> GAMSRQANRGTESKKMSSELFTLTYGALVTQLCKDYENDEDVNKQLDRMGYNIGVRLIEDFLARSNVGRCHDFRETADVIAKVAFKMYLGITPSITNWSPAGDEFSLILENNPLV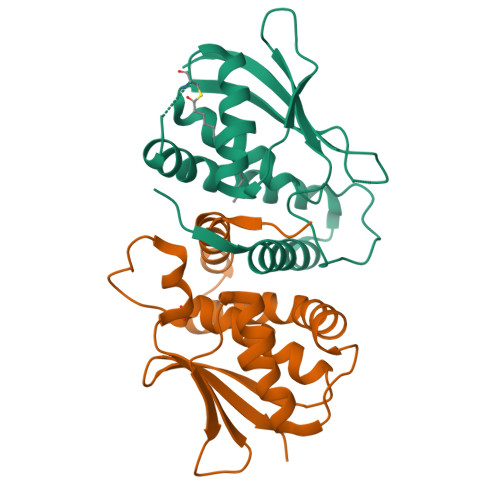DFVELPDNHSALIYSNLLCGVLRGALEMVQMAVEAKFVQDTLKGDGVTEIRMRFIRRIEDNLPAGEE;> PKTEVSVSAFALLFSEMVQYCQSRVYSVSELQARLADMGQGVGASLLDVLVMREKNGKRETKVLNILLFIKVNVWKALFGKEADKLEQANDDDKTYYIIEKEPLINAYISVPKENSTLNCAAFTGGIVEAILTHSGFPAKVTVHWHKGTTLMIKFDE>AYTTFSQTKNDQLKEPMFFGQPVNVARYDQQKYDIFEKLIEKQLSFFWRPEEVDVSRDRIDYQALPEHEKHIFISNLKYQTLLESIQGRSPNVALLPLISIPELETWVETWAFSETIHSRSYTHIIRNIVNDPSVVFDDIVTNEQIQKRAEGISSYYDELIEMTSYWHLLGEGTHTVNGKTVTVSLRELKKKLYLCLMSVNALEAIRFYVSFACSFAFAERELMEGNAKIIRLIARDEALHLTGTQHMLNLLRSGADDPEMAEIAEECKQECYDLFVQAAQQEKDWADYLFRDGSMIGLNKDILCQYVEYITNIRMQAVGLDLPFNTRSNPIPWINTWLVSDNVQVAPQEV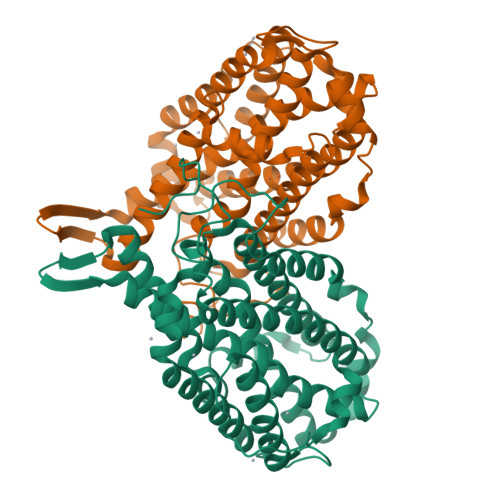EVSSYLVGQIDSEVDTDDLSNFQL[2x]>[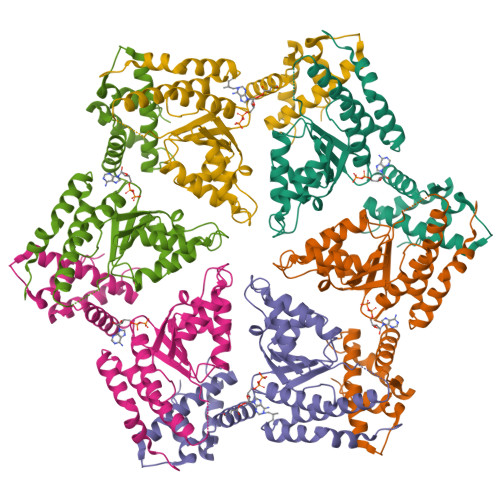6x]PTSIDLRAEYEGSGAKEVLEELDRELIGLKPVKDRIRETAALLLVERARQKLGLAHETPTLHMSFTGNPGTGKTTVALKMAGLLHRLGYVRKGHLVSVTRDDLVGQYIGHTAPKTKEVLKRAMGGVLFIDEAYYLYRPDNERDYGQEAIEILLQVMENNRDDLVVILAGYADRMENFFQSNPGFRSRIAHHIEFPDYSDEELFEIAGHMLDDQNYQMTPEAETALRAYIGLRRNQPHFANARSIRNALDRARLRQANRLFTASSGPLDARALSTIAEEDIRASRVFKGG> GAMNSSNYAELFNNDIKLFVDDTNVYRVTVHKTFEGNVATKAINGCIFTLNPKTGHLFLKIIHTSVWAGQKRLSQLAKWKTAEEVSALVRSLPKEEQPKQIIVTRKAMLDPLEVHMLDFPNIAIRPTELRLPFSAAMSIDKLSDVVMKATEPQMVLFNIYDDWLDRISSYTAFSRLTLLLRALKTNEESAKMILLSDPTITIKSYHLWPSFTDEQWITIESQMRDLILTEYGRKYNVNISALTQTEIKDIILGQNIKAPSVKRQKMAELEAARSEKQNDEEAAGASTVMKTKTINAQGEEIVVVASADYESQTFSSK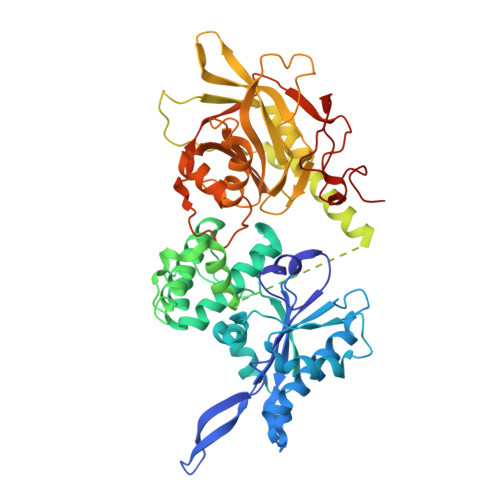NEWRKSAIANTLLYLRLKNIYVSADDFVEEQNVYVLPKNLLKKFIEISDVKIQVAAFIYGMSAKDHPKVKEIKTVVLVPQLGHVGSVQISNIPDIGDLPDTEGLELLGWIHTQTEELKFMAASEVATHSKLFADKKRDCIDISIFSTPGSVSLSAYNLTDEGYQWGEENKDIMNVLSEGFEPTFSTHAQLLLSDRITGNFIIPSGNVWNYTFMGTAFNQEGDYNFKYGIPLEFYNEMHRPVHFLQFSE> GPYIKRVIIKGFKTYRNETIIDNFSPHQNVIIGSNGSGKSNFFAAIRFVLSDDYSNLKREERQGLIHQGSGGSVMSASVEIVFHDPDHSMILPSGVLSRGDDEVTIRRTVGLKKDDYQLNDRNVTKGDIVRMLETAGFSMNNPYNIVPQGKIVALTNAKDKERLQLLEDVVGAKSFEVKLKASLKKMEETEQKKIQINKEMGELNSKLSEM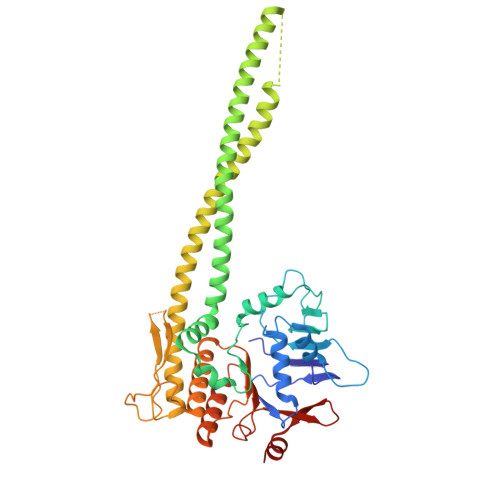EQERKELEKYNELERNRKRAFENFKKFNERRKDLAERASELDESKDSIQDLIVKLKQQKVNAVDSTFQKVSENFEAVFERLVPRGTAKLIIHRYTGVSISVSFNSKQNEQLHVEQLSGGQKTVCAIALILAIQMVDPASFYLFDQIDAALDKQYRTAVATLLKELSKNAQFICTTFRTDMLQVADKFFRVKYENKISTVIEVNREEAIGFIR> SLSNKLTLDKLDVKGKRVVMRVDFNVPMKNNQITNNQRIKAAVPSIKFCLDNGAKSVVLMSHLGRPDG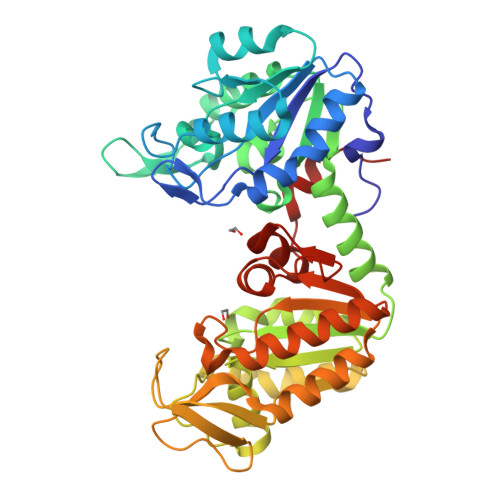VPMPDKYSLEPVAVELKSLLGKDVLFLKDCVGPEVEKACANPAAGSVILLENLRFHVEEEGKGKDASGNKVKAEPAKIEAFRASLSKLGDVYVNDAFGTAHRAHSSMVGVNLPQKAGGFLMKKELNYFAKALESPERPFLAILGGAKVADKIQLINNMLDKVNEMIIGGGMAFTFLKVLNNMEIGTSLFDEEGAKIVKDLMSKAEKNGVKITLPVDFVTADKFDENAKTGQATVASGIPAGWMGLDCGPESSKKYAEAVTRAKQIVWNGPVGVFEWEAFARGTKALMDEVVKATSRGCITIIGGGDTATCCAKWNTEDKVSHVSTGGGASLELLEGKVLPGVDALSNI>UUUUUAAUGAAGCCACAGGCCUGUGAGGGUCCUAAGCCCCUAAUUCAGAAGGGAAA[3x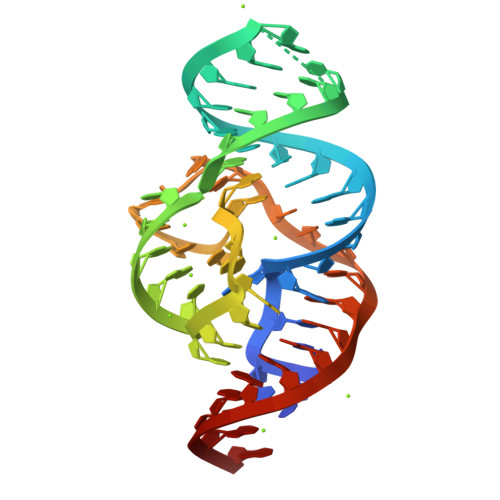]> GPMEKYREIHQRVRDLAPGTVSALECIDLLDRLYAVRHDLVDQMIKHDWSDNKDVERPIGQVLLMAGIPNDIIQGMEKKIIPNS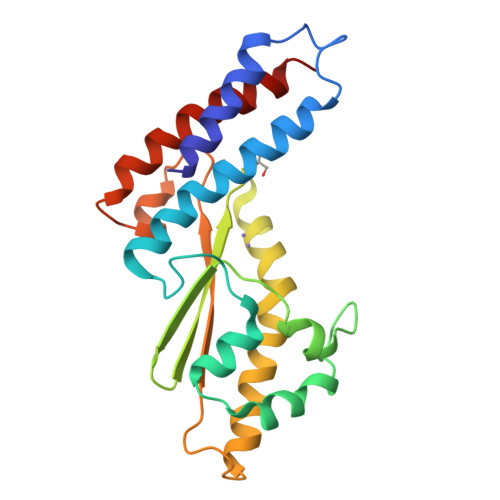PSGQVLKSFFRMTPDNYKITGNLIEFIEVTVTADVSRGIREAKIKYEGGLQFVEHLLETESRKGNIPQPYKITFSVVAVKTDGSNISTQWPSRRNDGVIQHMRLVQADINYVREHLIK> MSRKDYVLFDINTKAFVYGYQTNAIQRMLDFDYVCKRSSPSISAIINPSRAGIHKAFWGTKEIILPMYKTIPLAALAYPEADVMVNFASHRSAFETTMEALKEDTIRIVAVIAEGVPERQSRVMAATARKLDKIVIGPATVGGMTAGAFRIGNTAGTIENIIASKLYRPGCVGFVSKSGGMLNEAFNIISRNSDGIYEGVAIGGDRYPGSNMLDHILRYERNPAIKMIACLGELGGEDEYMIIQALKEKKITKPLVAWVTGTCSPYLPASVQFGHAGAKANTEKETAQAKNDAFRQAGAYVPRSFDDYGEMVRQVYDMLLTRGIVQKFDEPEVPRIPTDYSKALATGDIRKPTTFICTISDDSGEELLYA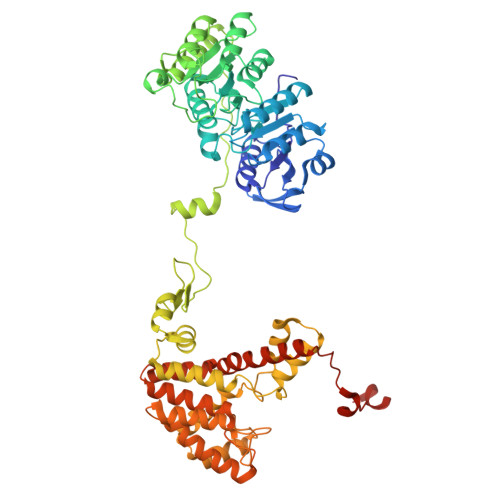GKKLSDVLDRKMGIGGVIGLLWFKKELPEYAAHFIELVIQIVADHGPAVSGAHNAIVASCAGKDLISSLCSGLLTIGPRFGGAIDDAAREFKRAQETGLAPEQFVGEMKKKGINIPGIGHKIKSVKNPDKRVQLLISYARANFPSTELLNYALQVEELTTAKKGNLILNVAGCIGILFIDLMSSCGAFSKEEIDEVVRLGYLNGLFALGRSIGLIGHILDQKRLGSRLYRHPAEDIAYMMPSEEEIQCKRDRGGSHHHHHH>[3x]ASTKAQPTEVSSILEERIKGVSDEANLNETGRVLAVGDGIARVFGLNNIQAEELVEFSSGVKGMALNLEPGQVGIVLFGSDRLVKEGELVKRTGNIVDVPVGPGLLGRVVDALGNPIDGKGPIDAAGRSRAQVKAPGILPRRSVHEPVQTGLKAVDALVPIGRGQRELIIGDRQTGKTAVALDTILNQKRWNNGSDESKKLYCVYVAVGQKRSTVAQLVQTLEQHDAMKYSIIVAATASEAAPLQYLAPFTAASIGEWFRDNGKHALIVYDDLSKQAVAYRQLSLLLRRPPGREAYPGDVFYLHSRLLERAAKLSEKEGSGSLTALPVIETQGGDVSAYIPTNVISITDGQIFLEAELFYKGIRPAINVGLSVSRVGSAAQVKALKQVAGSLKLFLAQYREVAAFAQFGSDLDASTKQTLVRGERLTQLLKQNQYSPLATEEQVPLIYAGVNGHLDGIELSRIGEFESSFLSYLKSNHNELLTEIREKGELSKELLASLKSATESFVATF;>[3x]ASAAQSTPITGKVTAVIGAIVDVHFEQSELPAILNALEIKTPQGKLVLEVAQHLGENTVRTIAMDGTEGLVRGEKVLDTGGPISVPVGRETLGRIINVIGEPIDERGPIKSKLRKPIHADPPSFAEQSTSAEILETGIKVVDLLAPYARGGKIGLFGGAGVGKTVFIQELINNIAKAHGGFSVFTGVGERTREGNDLYREMKETGVINLEGESKVALVFGQMNEPPGARARVALTGLTIAEYFRDEEGQDVLLFIDNIFRFTQAGSEVSALLGRIPSAVGYQPTLATDMGLLQERITTTKKGSVTSVQAVYVPADDLTDPAPATTFAHLDATTVLSRGISELGIYPAVDPLDSKSRLLDAAVVGQEHYD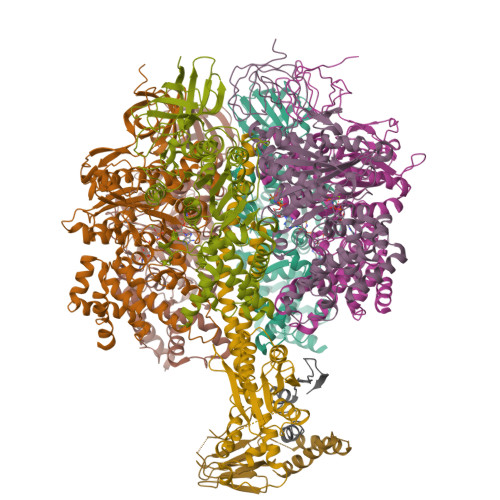VASKVQETLQTYKSLQDIIAILGMDELSEQDKLTVERARKIQRFLSQPFAVAEVFTGIPGKLVRLKDTVASFKAVLEGKYDNIPEHAFYMVGGIEDVVAKAEKLAAEAN;> ATLKEVEMRLKSIKNIEKITKTMKIVASTRLSKAEKAKISAKKMDEAEQLFYKNAETKNLDVEATETGAPKELIVAITSDKGLCGSIHSQLAKAVRRHLNDQPNADIVTIGDKIKMQLLRTHPNNIKLSINGIGKDAPTFQESALIADKLLSVMKAGTYPKISIFYNDPVSSLSFEPSEKPIFNAKTIEQSPSFGKFEIDTDANVPRDLFEYTLANQMLTAMAQGYAAEISARRNAMDNASKNAGDMINRYSILYNRTRQAVITNELVDIITGASSLG;> AEAAAASSGLKLQFALPHETLYSGSEVTQVNLPAKSGRIGVLANHVPTVEQLLPGVVEVMEGSNSKKFFISGGFATVQPDSQLCVTAIEAFPLESFSQENIKNLLAEAKKNVSSSDAREAAEAAIQVEVLENLQSVLK;> SAWRKAGMSYAAYLNVAAQAIRSSLKTELQTASVTNRSQTDAFYTQYKNGTAASEPTPMTK;>MQLVLAAKYIGAGISTIGLLGAGIGIAIVFAALINGVSRNPSIKDTVFPMAILGFALSEATGLFCLMVSFLLLFGV[10x]> NNRPEEANRIGLNTTIKGSLIGGDHTDVYTFNVASAKNIDISVLNEYGIGMTWVLHHES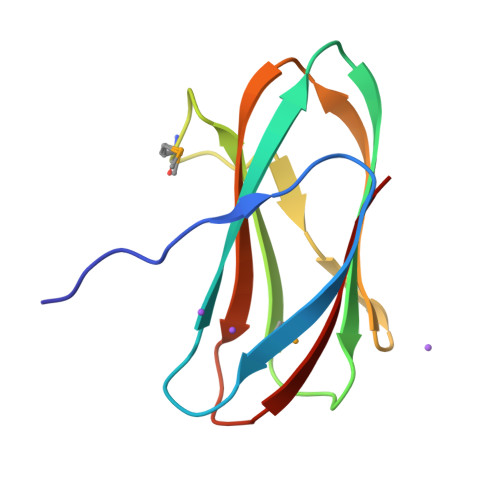DMQNYAAYGQANGNHIEANFNAKPGKYYLYVYKYDNGDGTYELSVK>[4x]GSHHKAVLAVRREDVNAWERRAPLAPKHIKGITNLGYKVLIQPSNRRAIHDKDYVKAGGILQEDISEACLILGVKRPPEEKLMSRKTYAFFSHTIKAQEANMGLLDEILKQEIRLIDYEKMVDHRGVRVVAFGQWAGVAGMINILHGMGLRLLALGHHTPFMHIGMAHNYRNSSQAVQAVRDAGYEISLGLMPKSIGPLTFVFTGTGNVSKGAQAIFNELPCEYVEPHELKEV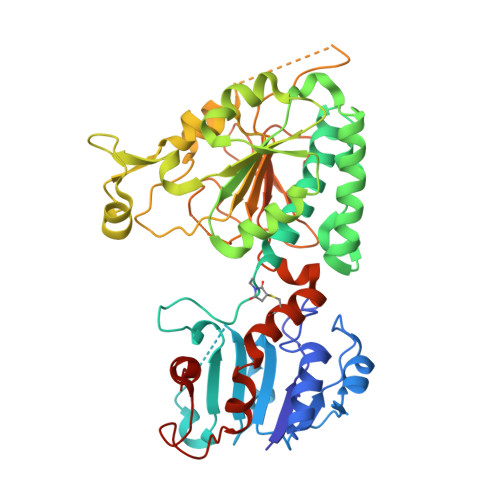SQTGDLRKVYGTVLSRHHHLVRKTDAVYDPAEYDKHPERYISRFNTDIAPYTTCLINGIYWEQNTPRLLTRQDAQSLLAPGKFSPAGVEGCPALPHKLVAICDISADTGGSIEFMTECTTIEHPFCMYDADQHIIHDSVEGSGILMCSIDNLPAQLPIEATECFGDMLYPYVEEMILSDATQPLESQNFSPVVRDAVITSN>[4x]MLGTSGVKIHPNGNSNQLGVQLENVKLTSLFKKLDKRCSLASWIKENIKKKECCFYVEDGREGICKCGYPKVQHCDEAIKPEDYMGEQWDKHRHVRETPTDAFGDISFGGLGQKTGKYVRVSSDTSCENLYQLMTEQWKLRSPNLLISVTGGAKNFYIKTHLKDKFRRGLIKVAQTTGAWILTGGTHAGVMKHVGMAVRDYTLSSGSMEGQIVVIGVAPWGVIHNRSTLIHPEGRFPAYYSLDEQGQGRLSCLDINHTHFLLVDDGTQGHYGVEIELRARLEKLISKLSLGNRESGVTIPVVCVVLDGGPGTLNTIYNSMLNHTPCVVLEGSGRLADVIAHVASVPVSKVTMALINRLLKRFFMQEYKNFTELQIIEWTKKIQDILRMPHLLTVFRIDEDKNYDVDVAILQALLKASRSDEHAGRHCWERQLELAVAWNRVDIAESEIFTEESQWTSSDLHPAMFSALVGDKPEFVRLLLENGVCVREFLEREETLCELYSHLPSCFFLRKLAKRVQGGKMRRGQEPLPGSRKVCLSHVSEEVRHLLGSFTQPLYIASRYKPTKDDVRLKVPSKGALDLPCSGEEWSADTVWDPGRDLFLWAVVQNNRELAEIGWEQCRDCIAAALAASKILRKLAQESGED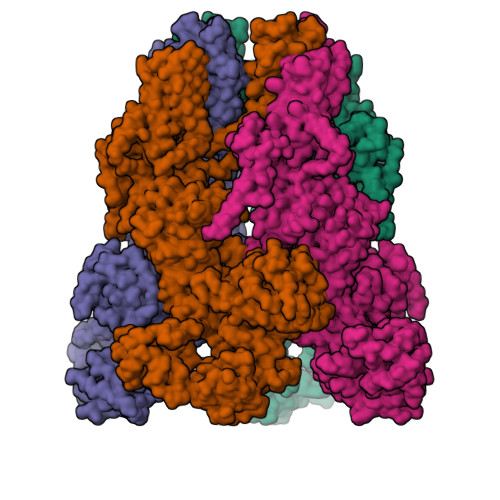DSEEATEMLELANHYEKQAIGVFSECHSWDAQRAQKLLIRISPSWGRSTCLWLALEAHDKSFIAHSGVQALLTQIWCGELSVDNPHWKVLLCMIFFPLIYTGFLTFRRDEDIQRQAERTEQQKLAMESVFAGQSDGKIKRHLRGFSQKSELKPLNCSSRLMSFLKSPQVKFYWNIASYFGFLWLFAVVLMIDFQTSPSWRELLLYVWLTSLVCEEIRQLYHDFDGSGFRRKAKMYIKDLWNILDVLSIVLFIAGLICRLQASDTVFYIGKVILCIDFIIFCLRLMAIFSISRTLGPKIIIVRRMMLDLFFFMFLLSIWVVAYGVAKQGILIENEERLNWIIRGAVYEPYITIFGNFPTNIDNTLFDISSCSVNASDPLKPKCPMLNADNTPVFPEWLTIMMLCVYLLFANILLLNLLIAIFNYTFQEVQDNTDTIWKFQRYELIKEYHSRPALPPPFILLSHLILFIRGVFLRDLPQRHKNFRQELEQTEEEELLSWEAYMKDNYLASTRQDESQSVEHRIHDTAEKVGAMSELLEREQEMVSATMAKRLARLEEQVSESAKALRWIIDALKSQGCKSKVQPPLMRSKSSDRDDGDSSGQETDDEEAPHMFARQLQYPDSTVRRFPVPEEKVSWEVNFSPYQPPVYNQQDSSESDTSALDKHRNPGGRTGIRGKGALNTLGPNHILHPIFTRWRDAEHKVLEFLAVWEDAEKRWALLGGPAQPDEPLAQVLERILGKKLNEKTKTLLKAGEEVYKGYVDDSRNTDNAWVETSIITLHCDKNTPLMADLNHMVESSLSSHQPLQWREVSSDACRCSYQREALRQIAHHHNTYF> HHHHHHAPAFRYTRSQSFDIFDINQKCFVLESPTQLVALHLQGPSSSQKVRLNIALYRPRGPRGSAGTGQMPVALGIKGYKLYMSCVMSGTEPTLQLEEADVMRDIDSVELTRFIFYRLDSPAEGTTRFES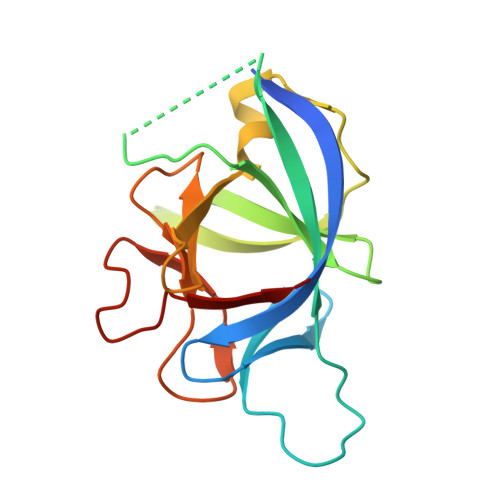AAFPGWFICTSLQPRQPVGITNQPDQVNIATYKLSGR> MSPYSSDTTPCCFAYIARPLPRAHIKEYFYTSGKCSNPAVVFVTRKNRQVCANPEKKWV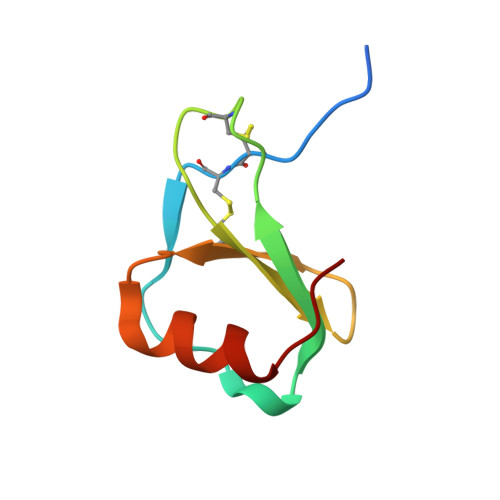REYINSLSMS>QGFEFNIMVVGQSGLGKSTLINTLFK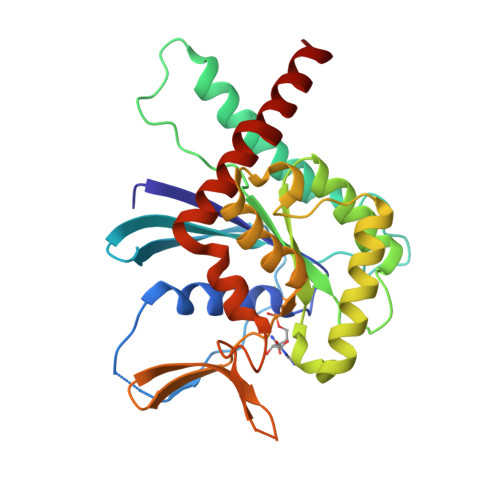SKISRKSVQPTSEERIPKTIEIKSITHDIEEKGVRMKLTVIDTPGFGDHINNENCWQPIMKFINDQYEKYLQEEVNINRKKRIPDTRVHCCLYFIPATGHSLRPLDIEFMKRLSKVVNIVPVIAKADTLTLEERVHFKQRITADLLSNGIDVYPQKEFDEDSEDRLVNEKFREMIPFAVVGSDHEYQVNGKRILGRKTKWGTIEVENTTHCEFAYLRDLLIRTHMQNIKDITSSIHFEAYRVKRLNEG[2x]> SNAMKQLSGLLGELRQKLCAGFPEQAGIQQLIFPAPGLVGRQLLEWLTAQTHFPQFYWRHRDNHEEAAVCGQTRSFADMKDADDFIQQNPDANGLRIWGLNAFEPVMVFGQLTDNGLVSGKNAQASFLFLPRLEILRRGKKTSLTLNLSSETSLQKDALQAITFIDQLMAARALPVLNARIQHSSHTPGYPQWRNLIQQALNDIEQQKLDKVVLARTTTLTLNKPLSCAAFMAASRQVNHRCYHFMLRFDDRQAFLGSSPERLYLRQQLHLETEALAGTVSNLDSDPQAAVLADWLMHDEKNQRENLLVVDDICQRLQGGVTAVDVMPPEIIRLRKVQHLR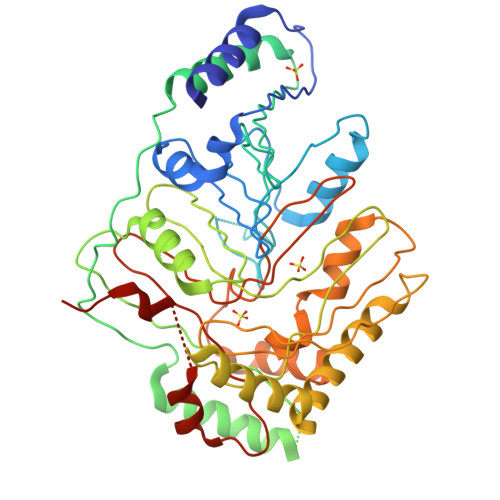RRICAQLSRASDTDCLQRLQPTAAVAGLPREAARQFIAKHELFSRGWYAGSAGYLSLKRTEFSVALRSARVDGQQIHLYAGAGIVAGSDAEQEWQEIDNKSAGLQSLLEHEAQPVKA oxadiazon 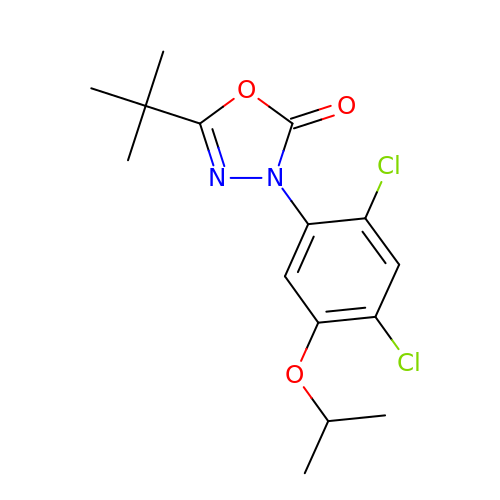| C15 H18 Cl2 N2 O3 | CHNUNORXWHYHNE-UHFFFAOYSA-N pmcMarE is a bacterial enzyme that catalyzes a unique 2-oxindole production reaction through monooxygenation of (2S,3S)-β-methyl-l-tryptophan (β-Me-l-Trp). The amino acid sequence of MarE shares significant similarity with tryptophan 2,3-dioxygenase (TDO), a histidine-ligated heme-dependent enzyme that catalyzes the activation and insertion of molecular oxygen by a histidine-ligated heme into the indole ring of l-tryptophan (l-Trp), producing N-formylkynurenine (NFK). TDO and its closely related homolog, indoleamine 2,3-dioxygenase (IDO), catalyze stepwise O-atom transfers, completing dioxygenation through two sequential monooxygenation reactions. However, MarE diverges functionally by catalyzing only a single monooxygenation reaction on a tryptophan metabolite, terminating the oxidation process before full dioxygenation. To elucidate its enzyme-substrate interaction mode, we present the first X-ray crystal structures of MarE in complex with its prime substrate, (2S,3S)-β-methyl-l-tryptophan and cyanide at 1.89 Å resolution as well as a truncated yet catalytically active version in complex with the substrate at 2.45 Å resolution. These structures establish MarE as a member of the heme-dependent aromatic oxygenase (HDAO) superfamily and reveal its evolutionary link to indoleamine 2,3-dioxygenase (IDO) and tryptophan 2,3-dioxygenase (TDO).

MarE C280S crystals were obtained by crystallization in the presence of 50 mM sodium cyanide and 10 mM β-Me-l-Trp. The MarE C280S crystal belongs to a primitive monoclinic space group of P21 and contains four protomers in an asymmetric unit. The structure determined at 1.89-Å resolution forms a dimer of dimers, consistent with the homo-tetrameric oligomeric state of MarE in the solution state, without requiring further crystallographic symmetry operations. Each monomer consists of ten α-helices, with a disordered region spanning residues of 217 to 226. Conversely, in the 1.89-Å ternary complex structure with full-length (1–284) MarE C280S, the β-Me-l-Trp is unambiguously assigned, with the substrate amino group oriented toward the heme center and the β-methyl group directed toward the hydrophobic pocket in all four subunits. The substrate amino group is oriented towards the heme center, interacting with the main-chain carbonyl oxygen of Ala125 and the nitrogen of cyanide. The cyanide nitrogen, in turn, interacts with the main-chain nitrogen of Gly127, both of which are part of the DATG loop originating from the lid helix α5 and extending through the active site. The carboxylate group of the substrate interacts with Nε of Arg118 from the lid helix α5 and the main-chain nitrogen of Leu232, a component of the SLGGR loop. Residues from the neighboring subunit, including Tyr24∗, Val27∗, and Leu28∗, along with Phe51 and Leu121, create a deep hydrophobic pocket that accommodates the indole ring of β-Me-l-Trp.

>[4x]GHMKRSLNPDEPNALLSYDFDRGSNYENVLHLTDALGALVPESETEHPDQRFFQVTHLITEYAWVQVHYELRRAIGHLDEDRYHQAVRMFDRATGLSEVTVQAVRLLTDHLPQHSLLMMRNALPEDATGLDSPGYRNLRRVARPVWKAYEQAVERAGLSLQDVIAQQDDGYDGPRSGGSQSLALVREAMLRLDGSVLGWKQHHLIMVWSQLGGQPGLRKGNEEGDDGLELPQSLGGRSLATLEARSQLALFPELWRAAEDAYWLLGTRHDTDAPVRGGGNGSPVQH>[8x]MGSSHHHHHHSSGPQQGLRHLLSAGEIWISPQGNDLNDGTRPSPKATLTSALRQAREWRRTDDERVRGGITICMEGGTYALYEPVFIRPEDSGTEDSPTVIRPVADEKVVLSGGIRIGGWKKQGKLWVADVPMFNGRPLDFRQLWVNGKKAVRARDVEDFEKMNRICSVDEKNEILYVPAVAIRRLVDGKGALKAKYAEMVLHQMWCVANLRIRSVELAGDSAAIRFHQPESRIQFEHPWPRPMVTTDGHNSAFYLTNARELLDVAGEWYHDIDARKVYYYPREGEKLQDAGTEVIVPAIETLIQVKGTFDRPVSHIRFEKITFSHTTWMRPSEKGHVPLQAGMYLTDGYRIDPKMERDYLNHPLDNQGWLGRPAAAVSVAAANQIDFERCRFDHLGSTGLDYEEAVQGGVVRGCLFRDIAGNGLVVGSFSPAAHETHLPYDPTDLREVCAHQQISNCYF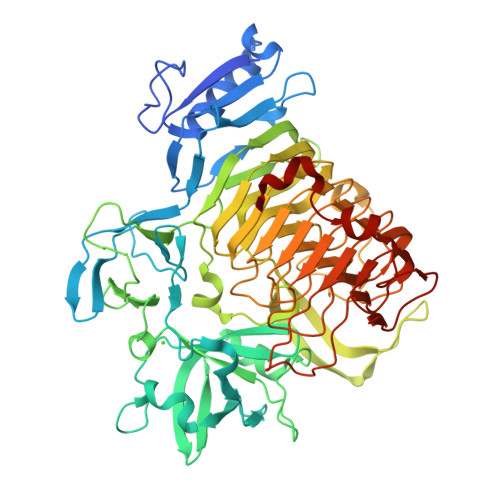TEVGNEDWGCLAILAGYVKDINIEHNEICEVPYSGISLGWGWTQTVNCMRNNRVHANLIHHYAKHMYDVAGVYTLGSQPKSYVTENCVHSIYKPGYVHDPNHWFYLYTDEGSSFITVRDNWTEGEKYLQNANGPGNVWENNGPQVDTVIRERAGLEAEYRDLKK> MAANKSKGQSSLALHKVIMVGSGGVGKSALTLQFMYDEFVEDYEPTKADSYRKKVVLDGEEVQIDILDTAGLEDYAAIRDNYFRSGEGFLLVFSITEHESFTATAEFREQILRVKAEEDKIP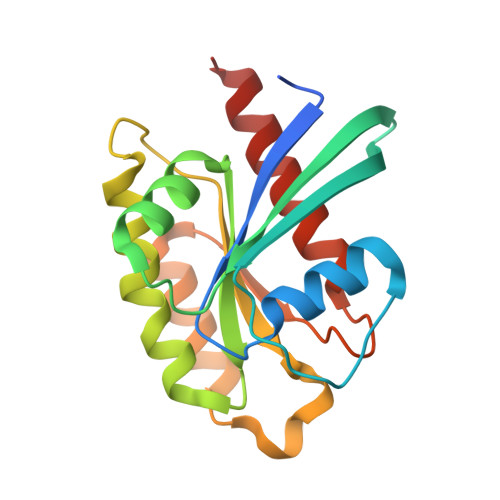LLVVGNKSDLEERRQVPVEEARSKAEEWGVQYVETSAKTRANVDKVFFDLMREIRTKKMSENK>GESNQQIADFDKEKATLDEADIDERMKLAQAFNDSLNNVVSGDPWSEEMKKKGRAEYARMLEIHERMGHVEIPVIDVDLPVYAGTAEEVLQQGAGHLEGTSLPIGGNSTHAVITADTGLPTAKMFTDLTKLKVGDKFYVHNIKEVMAYQVDQVKVIEPTNFDDLLIVPGHDYVTLLTCTPYMINTHRLLVRG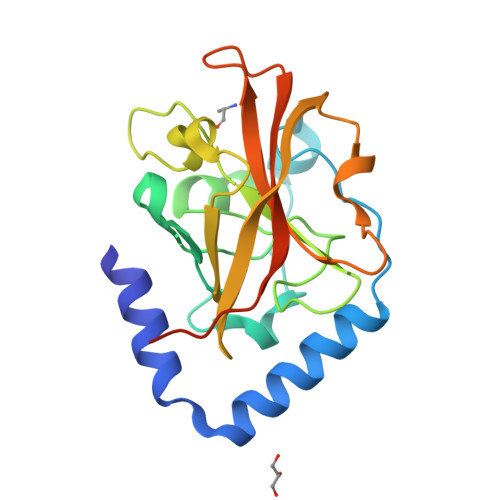HRIPYVAEVEEEFIAANKLSH[2x]> MGRAAEVPGPEPG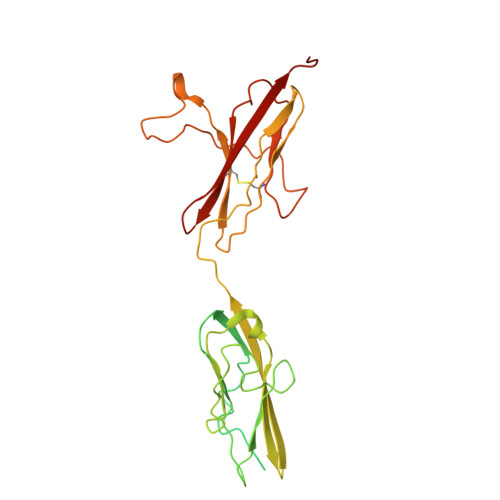QQEQLVFGSGDAVELSCPPPGGGPMGPTVWVKDGTGLVPSERVLVGPQRLQVLNASHEDSGAYSCRQRLTQRVLCHFSVRVTDAPSSGDDEDGEDEAEDTGVDTGAPYWTRPERMDKKLLAVPAANTVRFRCPAAGNPTPSISWLKNGREFRGEHRIGGIKLRHQQWSLVMESVVPSDRGNYTCVVENKFGSIRQTYTLDVLERSPHRPILQAGLPANQTAVLGSDVEFHCKVYSDAQPHIQWLKHVEVNGSKVGPDGTPYVTVLKTAGANTTDKELEVLSLHNVTFEDAGEYTCLAGNSIGFSHHSAWLVVLPAEEELVE>[2x]AVYTLPELPYDYSALEPYISGEIMELHHD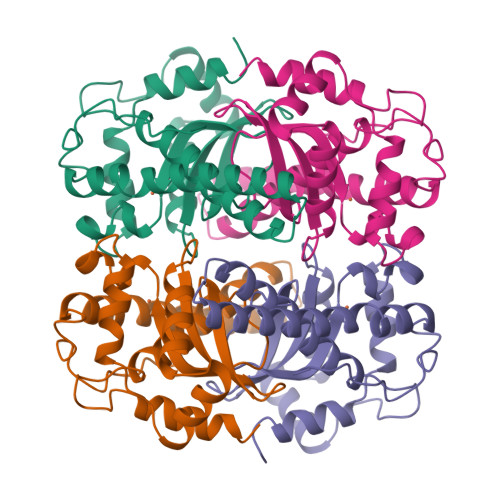KHHKAYVDGANTALDKLAEARDKADFGAINKLEKDLAFNLAGHVNHSVFWKNMAPKGSAPERPTDELGAAIDEFFGSFDNMKAQFTAAATGIQGSGWASLVWDPLGKRINTLQFYDHQNNLPAGSIPLLQLDMWEHAFYLQYKNVKGDYVKSWWNVVNWDDVALRFSEARVA>[4x]GPDDPLVINGEIEIVTRAPTPAHLADRFDEIRSGWTFRTDDTQALEMDDFENSGMVFVEEARAVWDRPEGTEGKACADCHGAVDDGMYGLRAVYPKYVESAGKVRTVEQMINACRTSRMGAPEWDYIGPDMTAMVALIASVSRGMPVSVAIDGPAQSTWEKGREIYYTRYGQLDLSCASCHEQYFDHYIRADHLSQGQINGFPSYRLKNARLNAVHD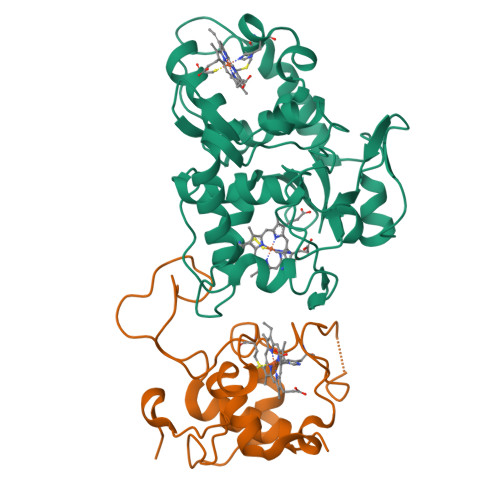RFRGCIRDTRGVPFAVGSPEFVALELYVASRGNGLSVEGPSVRN;>AEVAPGDVAIDGQGHVARPLTDAPGDPVEGRRLMTDRSVGNCIACHEVTEMADAQFPGTVGPSLDGVAARYPEAMIRGILVNSKNVFPETVMPAYYRVEGFNRPGIAFTSKPIEGEIRPLMTAGQIEDVVAYLMTLTQ[4x]>SERFPNDVDPIETRDWLQAIESVIREEGVERAQYLIDQLLAEARKGGVNVAAGTGISNYINTIPVEEQPEYPGNLELERRIRSAIRWNAIMTVLRASKKDLELGGHMASFQSSATIYDVCFNHFFRARNEQDGGDLVYFQGHISPGVYARAFLEGRLTQEQLDNFRQEVHGNGLSSYPHPKLMPEFWQFPTVSMGLGPIGAIYQAKFLKYLEHRGLKDTSKQTVYAFLGDGEMDEPESKGAITIATREKLDNLVFVINCNLQRLDGPVTGNGKIINELEGIFEGAGWNVIKVMWGSRWDELLRKDTSGKLIQLMNETVDGDYQTFKSKDGAYVREHFFGKYPETAALVADWTDEQIWALNRGGHDPKKIYAAFKKAQETKGKATVILAHTIKGYGMGDAAKGKNIAHQVKKMNMDGVRHIRDRFNVPVSDADIEKLPYITFPEGSEEHTYLHAQRQKLHGYLPSRQPNFTEKLELPSLQDFGALLEEQSKEISTTIAFVRALNVMLKNKSIKDRLVPIIADEARTFGMEGLFRQIGIYSPNGQQYTPQDREQVAYYKEDEKGQILQEGINELGAGCSWLAAATSYSTNNLPMIPFYIYYSMFGFQRIGDLCWAAGDQQARGFLIGGTSGRTTLNGEGLQHEDGHSHIQSLTIPNCISYDPAYAYEVAVIMHDGLERMYGEKQENVYYYITTLNENYHM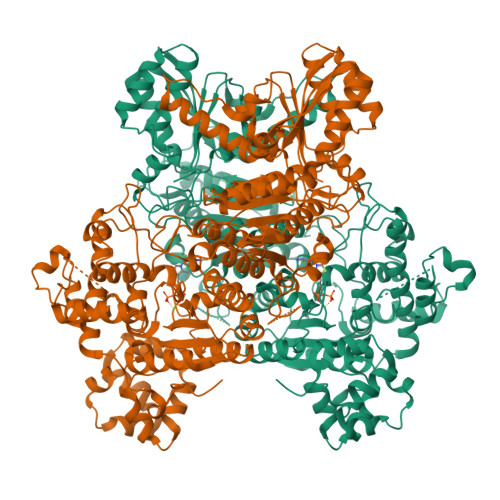PAMPEGAEEGIRKGIYKLETIEGSKGKVQLLGSGSILRHVREAAEILAKDYGVGSDVYSVTSFTELARDGQDCERWNMLHPLETPRVPYIAQVMNDAPAVASTDYMKLFAEQVRTYVPADDYRVLGTDGFGRSDSRENLRHHFEVDASYVVVAALGELAKRGEIDKKVVADAIAKFNIDADKVNPRLA[2x]>[2x]MGSDKIHHHHHHENLYFQGMSDIELLETLAGTDQPRVMATIIHVEGSSYRKEGAMMLFQEDGTQVGLLSGGCLETDLTIKAQKVWQEQLPRTVVYDLSSEDDLSWGQGSGCNGTISVLLEPVDLKLRQHLKRVYDYLCAGKSVFHVKKLSTSGAVLEYAFILDESVYFGEWHSGHPVEWIRKIDENEEPLMFTH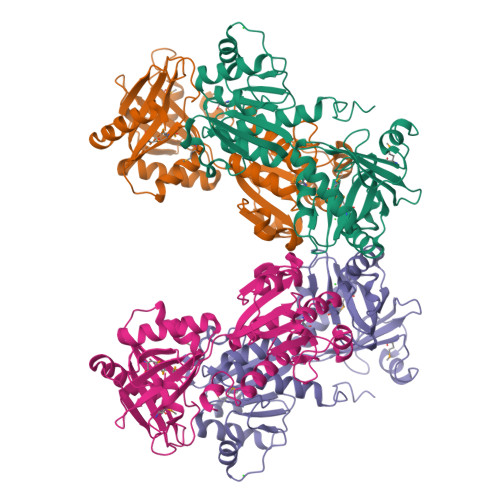IYSPKERLIIFGAGPDVPPLVTFASNVGFYTVVTDWRPNQCEKHFFPDADEIIVDFPADFLRKFLIRPDDFVLIMTHHFQKDQEILHFLLEKELRYIGILGSKERTRRLLQNRKPPDHLYSPVGLSIDAQGPEEIAISIVAQLIQLIRSRKQASSPFSYLFQPESCKH> HHHHHHIVIFVDFDYFFAQVEEVLNPQYKGKPLVVCVYSGRTKTSGAVATANYEARKLGVKAGMPIIKAMQIAPSAIYVPMRKPIYEAFSNRIMNLLNKHADKIEVASIDEAYLDVTNKVEGNFENGIELARKIKQEILEKEKITVTVGVAPNKIL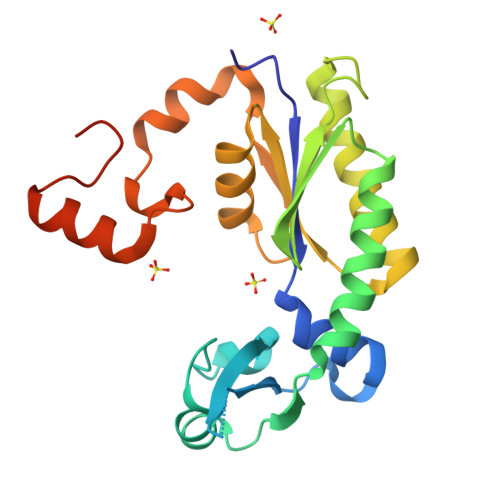AKIIADKSKPNGLGVIRPTEVQDFLNELDIDEIPGIGSVLARRLNELGIQKLRDILSKNYNELEK> GPLGSDLKDAEAVQKFFLEEIQLGEELLAQGDYEKGVDHLTNAIAVCGQPQQLLQVLQQTLPPPVF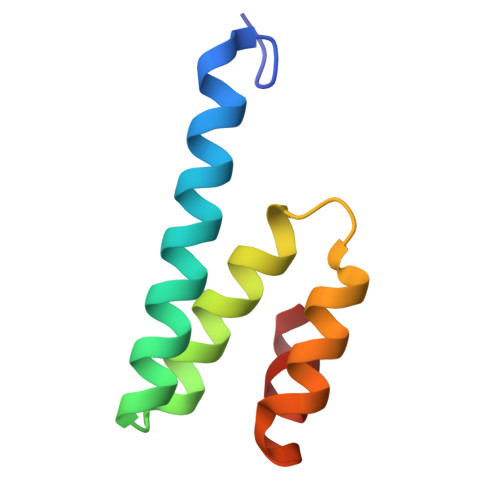QMLLTKL In the current study, we present the characterisation of an avidin-like protein in zebrafish, called zebavidin. Although zebavidin has many unique physicochemical and structural features, it clearly can be classified as a new member of the avidin protein family based on its structure and function. Structural and functional characterisation confirmed the hypothesis that zebavidin is a new member of the avidin protein family and binds tightly to biotin, even though the biotin-binding affinity of zebavidin is substantially lower than that measured for avidin or streptavidin. Zebavidin is an avidin-like protein from zebrafish and highly expressed in the gonads of adult fish but our preliminary results suggest that it is not critical for the development of the embryo.

The homotetramer of zebavidin resembles that of chicken avidin and is a typical “dimer of dimers”. Each of the 16 monomers in the asymmetric unit is structurally highly similar to each other and the Cα atoms of the monomers superimpose with a root mean square deviation (rmsd) of less than 0.3 Å; the tetramers superimpose with the same accuracy. The major structural differences are found at the biotin-binding loop, the L3,4-loop, which is three or more residues longer in zebavidin than in the other known avidin structures; the sequence and conformation of the L3,4-loop is also unique and especially affects the conformation of the adjacent L5,6-loop, which, in turn, is one amino acid shorter than in other avidin structures. The unique L3,4-loop and L5,6-loop affect the mode of biotin binding in zebavidin, even though most biotin-binding residues are conserved in zebavidin when compared to other avidins. In contrast, Glu38, Ser39, Thr40, Ala43, Ala44, Trp70, Ser74 and Leu98, which surround the valeric acid moiety of biotin, mostly have unique interactions. The L5,6-loop is shorter than in other avidins and a residue equivalent to Phe72 in avidin is missing, affecting the positioning and conformation of Lys72, which is not in direct contact with biotin even though the equivalent residue Ser73/Ser72 in avidin/xenavidin is hydrogen bonded to biotin. However, in zebavidin a structural water molecule is found at a position matching that of the side-chain oxygen atom of Ser73 of avidin suggesting that this water molecule, and at least two other structural water molecules near the valeric acid moiety, may be important for biotin binding (Figure 7A&C). The free and relatively polar Cys75 in nonpolar environment at the IF1,4 interface of zebavidin, together with several other unique interactions found at the same interface, may also weaken the quaternary structure, enabling transient oligomeric states under different buffer conditions.

>[16x]QTVSSCNVTGVWRNELGSTLRVKAEGSEVRGVYQTAVESTRGAAGHHRSARIIGMVSDGTQPTVSFSVLWEKGSCSAWVGQCFILDDGAQVLKTFWMLRSVADNLASAWGSTRMGEDIFFKTGVSN>MQQEQSYRIEKDFLGEKKIPADAYYGIQTLRATENFPITGYRIHEELIRALAMVKKAAALANMETKRLPAHIGEAIVAACDEIIAGQWHDQFIVDPIQGGAGTSINMNANEVIANRALEIMGKKKGDYFHVRPNSDVNMSQSTNDAFPTAVHIAVLTLLDHLLETMERMRDAFAEKAKAFDPYIKMGRIHLQDAVPIRLGQEFEAYTRVIERDIQRIKQSRGHLYEINMGATAVGTGLNADPRYIESVVKHLREISGYPLVGAENLVDATQNTDAYTEVSAALKVCMMNMSKIANDLRLMASGPRAGLGEITLPARQPGSSIIPGMVCPVMAEVINQIAFQVIGNDHTICLASEAGQLELNVMEPVLVFNLLQSISIMNNGFRVFTEYCVKGIEANEEKMKEYVEKSVGVITAVNPHIGYEVASRIAREATLTGQSVRDLCRKYDVLSDEELDLILDPYEMTHPGIAGASLLERD[2x]

Aspartate ammonia lyases catalyze the reversible amination of fumarate to l-aspartate. Furthermore, a conserved flexible loop, named SS-loop, that contains a two serine signature sequence plays an important role in substrate binding and catalysis. One of the serines acts as a general base in the deamination reaction by abstracting a proton from the Cβ atom of the substrate, forming an enolate anion intermediate. For this, the SS-loop changes from an open conformation in the absence of substrate to a closed conformation that covers the active site in the presence of substrate.

The resulting three variants equipped with the AspB-A1 pocket were well expressed and performed better in β-alanine synthesis than the corresponding variants with the A5 pockets. These results identified the variants BbAsp-A1+A424E, CcAsp-A1+A424S+I431T, and StAsp-A1+S421E as the best enzymes for β-alanine synthesis. For the sake of brevity, they were renamed BbAsp-5x, CcAsp-6x, and StAsp-5x, respectively. To rationalize the effect of mutations that allowed for β-alanine synthesis, crystal structures of variants AspB-6x and CcAsp-6x were determined to 1.9 and 3.1 Å resolution, respectively. While the wild-type AspB crystal structure contains both open and closed SS-loops, unliganded AspB-6x and CcAsp-6x adopted the typical closed conformation observed previously only in the liganded active sites of wild-type AspB. Importantly, the C2 carbon of acrylate is located in close proximity to Ser318-OH (Ser320 in CcAsp-6x), at a distance of ∼3 Å, which is suitable for its deprotonation during the reaction that results in the formation of β-alanine. In the CcAsp-6x variant, the SS-loop adopts a slightly different conformation as in AspB-6x, allowing the active site residues, including the catalytic serine, to more closely approach the substrate. This subtle difference in the SS-loop conformation may perhaps be related to the higher activity of the CcAsp-6x variant. A similar destabilizing effect on the open SS-loop conformation can be rationalized for the A424S and I431T mutations in CcAsp-6x. The inserted mutations allow for formation of hydrophobic contacts with acrylic acid and for positioning of this new substrate in the active site, both in the AspB variant AspB-6x and in the homologue CcAsp-6x. The latter was generated by the transplantation of activity-enhancing mutations into a homologous aspartase discovered after genome mining.> IPPIPPVDFAKYGEIEEVPMTRLMQIGATNLHRSWLNVPHVTQFESADITELEAFRVAQKAVAEKAGVKLTVLPLLLKACAYLLKELPDFNSSLAPSGQALIRKKYVHIGFAVDTPDGLLVPVIRN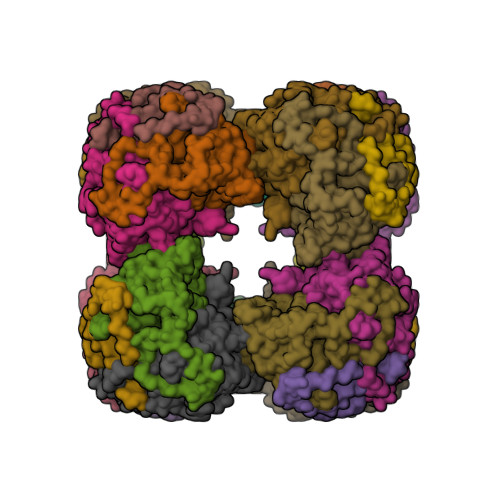VDQKSLLQLAAEAAELAEKARSKKLGADAMQGACFTISSLGHIGGTAFTPIVNAPEVAILGVSKASMQPVWDGKAFQPRLMLPLSLSYDHRVIDGAAAARFTKRLGDLLADIRAILL>[8x]MRT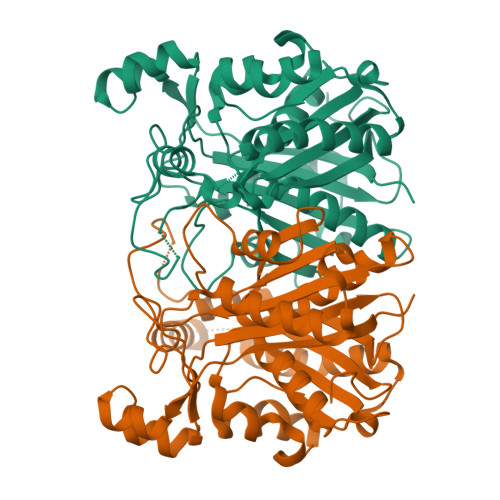PDIFIKATGRFLPETVSVEWAVEQGHYSAEDAELHELGGAAVAGDTPAPDMALWAAQQAVKRCGHRPEDLGLLLYVDSWHQGPDGWQPQYYLQRHLVGGDVLAVEIQQGCNGMFSALELAAAHLRAGPRPGSALVVAADNFGTPLFDRWTTGPGYIAGDGAGAVVLTTEPGFARLLAVRSLAVPEAEQMHRGAEPLFPPGATIGRPLNFTSRNAAFRELSLTEGLGTGALMRVHQRTLEVVEKTLSEAGITLGDITRVAYMNFSREIVEQRCMAALGLPMSASTWEFGRKLGHLGASDQVVALDELVTTGELGPGDHLLMLGMGPGVTLSCAVVKVLTPAPWSD> 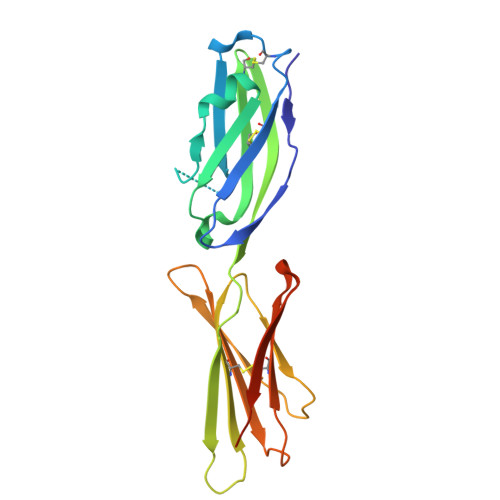LFTVTAPKEVYTVDVGSSVSLECDFDRRECTELEGIRASLQKVENDTSLQSERATLLEEQLPLGKALFHIPSVQVRDSGQYRCLVICGAAWDYKYLTVKVKASYMRIDTRILEVPGTGEVQLTCQARGYPLAEVSWQNVSVPANTSHIRTPEGLYQVTSVLRLKPQPSRNFSCMFWNAHMKELTSAIIDPLSRMEPKVPRT> GPLGSLCGRVFKVGEPTYSCRDCAVDPTCVLCMECFLGSIHRDHRYRMTTSGGGGFCDCG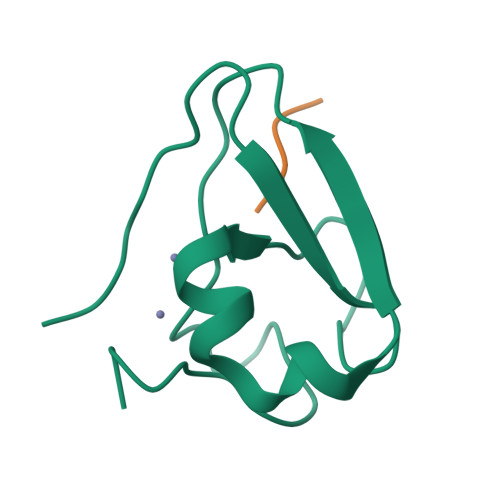DTEAWKEGPYCQKHEL;> RLWS> MATRTISCATASCLQSALKNAKPGDDIVLAEGVTFKGSFKAEASGTASQPITIRSAGSVNPAVLSGYSTGGGYSLYVTGDYWNITGLKMTGALKGIMLDHANHV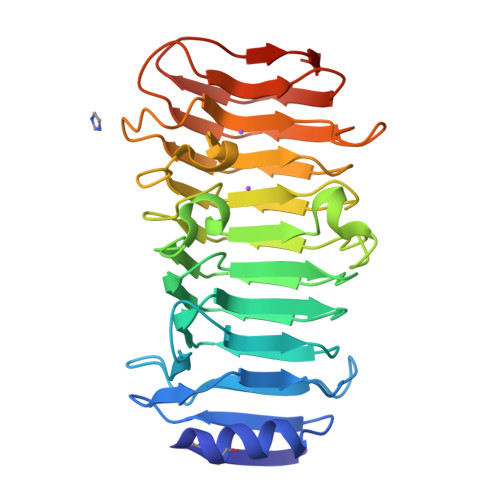QMDGLEIYDIGDEGVHFRDGSSDNIIRNSHIYNTGLIEAGFGEGIYVGSDKGKWATYNKSADRNVISGVRIGPGVAAEHIDIKEGTVGTIVENSVFNGTGITGANYADSFIDVKGNDAVIRNNIGYRNGNSNIVDAFQVHVQVAGWGQNATFTGNTVYLDQAAPYVVNAVGDATASAAGNQRYPAGNLYQGHVNALEHHHHHH> MEYKDTLLMPKTEFPMRGNLPNREPKMQEQWAEMNIYEKVQKRTEGRPLFVLHDGPPYANGDIHMGHALNKILKDFIVRYKSMSGFCAPYVPGWDTHGLPIETALTKNKKVNRKEMTVAEFRKLCEQYAWEQVNGQREQFKRLGVRGDWDNPYVTLQPQYEAQQIKVFGDMAKKGYIYKGLKPVYWSPSSESALAEAEIEYYDKRSASIYVAFNVKDGKGVLEQDEKFIIWTTTPWTMPANQGIAVNPELQYSVVEADGAKYVVATELIETVAKEIEWADYKTLRTVKGSELERVVAEHPIYKRDSLVVLGDHVTTDAGTGCVHTAPGHGEDDFIVGQKYGLEVLCPVDSKGHMTNEAPGFEGLFYDKANKPITDKLEEEGALLKLSFITHSYPHDWRTKKPTIFRATAQWFASIKDFREDLLKAVEKTKWVPTWGETRLYNMVRDRGDWCISRQRAWGVPIPVFYAENEEPIITDETIEHVSNLFREHGSNVWFEREAKDLLPEGFTHEGSPNGRFTKETDIMDVWFDSGSSHQAVLEEREDLQRPADLYLEGSDQYRGWFNSSLSTSVAVTGEAPYKGVLSHGFALDGEGRKMSKSLGNVVIPEKVMKQLGADILRLWVASVDYQADVRVSDNILKQVAEVYRKIRNTFRFLLGNLADFNPTTDAVAVEDLREVDRYMLVKLNKLIDKVKKSYDSYEFSSIYHAVHNFCTIDMSSFYLDFAKDVLYIEAENNVERRSIQTVLYETLLSLTKLVSPILSHTADEVWVHIPNVTEESVQLVDMPEVQEIEGADQLVEKWDAFMELRDEVLKALEQARNEKVIGKSLEAKLTLYPTADTKELLASISENVGQLFIVSDLEVAEGEAPAEAQKFSYASIVVSKAEGEKCERCWVVSPTVGEDQDHPTLCTRCADVVKNHYVQQ

Mupirocin, a clinically used natural antibiotic, inhibits isoleucyl-tRNA synthetase (IleRS), an enzyme that links isoleucine to its tRNAIle for protein synthesis. Two IleRSs, mupirocin-sensitive IleRS1 and resistant IleRS2, coexist in bacteria. Specifically, type 1 proteins (IleRS1) are strongly inhibited by mupirocin (Ki in low nanomolar range), while IleRS2, which are homologous to IleRSs from the eukaryote cytosol, exhibit resistance to mupirocin concentrations that are about three orders of magnitude higher. AARSs catalyze the formation of AA-tRNA in two steps within the same active site. The amino acid is first activated by ATP to form an aminoacyl-adenylate (AA-AMP) intermediate, followed by the transfer of the aminoacyl moiety to the tRNA.

To understand how IleRS2, but not IleRS1, accommodates the non-canonical motif, we used X-ray crystallography to determine the structures of a pair of IleRS enzymes from the same organism. Apart from wild-type PmIleRS1 and PmIleRS2, both of which harbor the canonical HXGH motif, we also structurally characterized their corresponding GXHH mutants, all in complex with a non-hydrolyzable analog of the isoleucyl-adenylate reaction intermediate, Ile-AMS. The insights into why IleRS2, but not IleRS1, can tolerate the non-canonical signature motif came from the crystal structures of the pair of PmIleRS1 and PmIleRS2, both in complex with Ile-AMS. However, superimposing the HUP catalytic cores of IleRS1 (residues 50–174 and 523–635) and IleRS2 (residues 40–168 and 513–632) unraveled conformational rearrangements within the signature motifs in the active sites. Relative to IleRS1, the KMSKS loop assumed a more closed conformation in IleRS2, as indicated by a 5.0 Å displacement of the first Lys backbone towards helix α1. No such ligand-dependent rearrangements in the HXGH motif are observed in PmIleRS1.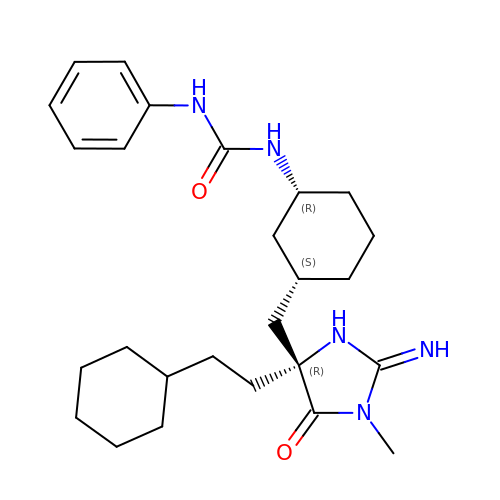1-[(1R,3S)-3-{[(2E,4R)-4-(2-cyclohexylethyl)-2-imino-1-methyl-5-oxoimidazolidin-4-yl]methyl}cyclohexyl]-3-phenylurea | C26 H39 N5 O2 | CVMRAJSOLFSMNH-UNIVCBNLSA-N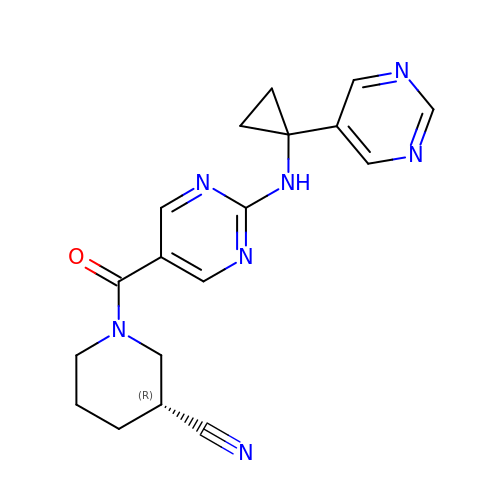(3R)-1-(2-{[1-(pyrimidin-5-yl)cyclopropyl]amino}pyrimidine-5-carbonyl)piperidine-3-carbonitrile | C18 H19 N7 O | CDTXEVWHMGPGKZ-ZDUSSCGKSA-N Bacillus subtilis can form structurally complex biofilms on solid or liquid surfaces, which requires expression of genes for matrix production. The transcription of these genes is activated by regulatory protein RemA, which binds to poorly conserved, repetitive DNA regions but lacks obvious DNA-binding motifs or domains. Here, we present the structure of the RemA homologue from Geobacillus thermodenitrificans, showing a unique octameric ring with the potential to form a 16-meric superstructure. These results, together with further biochemical and in vivo characterization of B. subtilis RemA, suggests that the protein can wrap DNA around its ring-like structure through a LytTR-related domain.

Previously, Winkelmann et al. reported another loss-of-function missense mutation of B. subtilis remA, named sor4, in which arginine 18 was changed into tryptophan (i.e., R18W32). In our structure of (Gt)RemA, arginine 18 localizes at the inner surface of (RemA)8. The guanidium moiety of arginine 18 of one RemA subunit forms a salt bridge and a hydrogen bond with the carboxyl moiety of aspartate 59 and the backbone carbonyl of alanine 17, respectively, both being from the adjacent RemA subunit. Thus, we decided to determine the structure of the (Gt)RemA-R18W variant. Thus, our structural analysis suggests that a major reason for the change of the 8-mer into a 7-mer is that tryptophan 18 is unable to interact with Asp59 and Ala17 of the neighboring subunit and thereby can no longer support the subunit orientation required for the stable formation of (RemA)8. An important consequence of the formation of (RemA-R18W)7 is that the arginines 50 and 51, which are crucial for DNA-interaction in the wildtype protein (see above), show a different spacing and orientation in the 7-mer. The observation that the RemA-R18W variant is still able to shift the PepsA promoter-containing DNA in an in vitro EMSA assay, but is clearly defective in vivo shows that the (RemA)8 is required to address a specific DNA topology to activate its target promoters.

>MGHHHHHHMMKFINIGYGNMVSAAWIITIVSPDSAPIKRIIQDAREKGKLVDATHGRRTRAVIITDSDHVILSSVQPETVANRLYGSDDFSEEG[7x]>MPLLDSFAVDHTRMQAPAVRTAKTMNTPHGDAITVFDLRFCIPNKEVMPEKGIHTLEHLFAGFMRDHLNGNGVEIIDISPMGCRTGFYMSLIGTPDEQRVADAWKAAMADVLKVQDQNQIPELNVYQCGTYQMHSLSEAQDIARHILERDV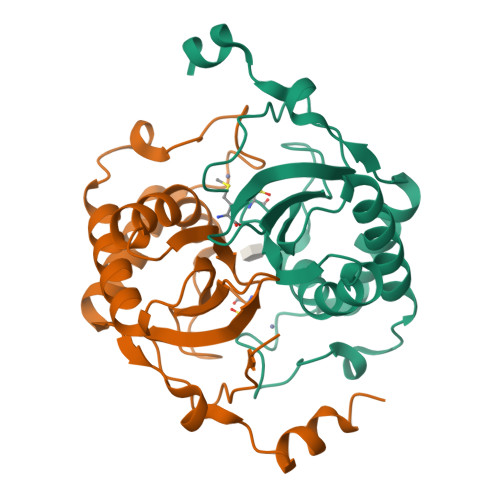RVNSNKELALPKEKLQELHILEHHHHHH[2x]> RPSGRKSSKMQAFRIWDVNQKTFYLRNNQLVAGYLQGPNVNLEEKIDVVPIEPHALFLGIHGGKMCLSCVKSGDETRLQLEAVNITDLSENRKQDKRFAFIRSDSGPTTSFES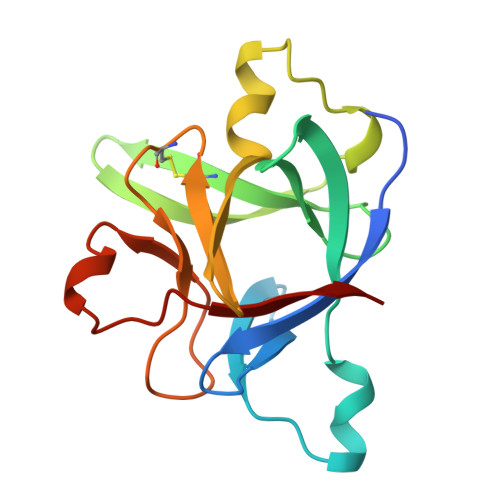AACPGWFLCTAMEADQPVSLTNMPDEGVMVTKFYFQEDE Anion exchanger 1 (AE1, band 3) is a major membrane protein of red blood cells and plays a key role in acid-base homeostasis, urine acidification, red blood cell shape regulation, and removal of carbon dioxide during respiration. AE1, a member of the solute carrier ion transport family 4 (SLC4), mediates the exchange of HCO3− with Cl− across plasma membranes. Mammalian erythrocyte AE1 is a ~100 kD integral transmembrane glycoprotein consisting of an N-terminal cytoplasmic domain (CD, residues 1 to 360 in human AE1) and a C-terminal trans-membrane domain (TMD, residues 361 to 911 in human AE1). Here we present the cryoEM structures of full-length bovine AE1 with its TMD captured in both IF and OF conformations.

The classes without CD and fully connected CD are both monomers in IF state. Particles from these two classes were combined and refined using a soft mask of the TM region. The final reconstruction of the IF state was resolved at 4.4 Å. The IF state features an elongated TM11, which incorporates residues from intracellular loop 5 (IL5) between TMs 10 and 11, and partially unfolded TM10. In contrast, the core domain shows a remarkable difference between the OF human and bovine AE1 on one hand and the IF bovine AE1 on the other hand. This difference comes from rigid rotation of the core domain ~20° with respect to the gate domain followed by diagonal downward displacement of the core with <5 Å along the z axis and small lateral motion in the XY plane. Further inspection of the IF structure of bovine AE1 TMD reveals that, due to the rotation and downward motion of the core domain, the ion coordination site becomes open to the cytoplasm and fully closed to the extracellular side, i.e., it is in the IF open state not previously observed in AE1. IL5 between TM10 and TM11, which assumes an antiparallel β-hairpin conformation in the OF state, loses this β-hairpin structure and part of it folds into the elongated α-helix of TM11 in the IF state. The concerted movement of TMs 10 and 11 and the β-hairpin to α-helix transition of IL5 opens a large cavity at the intracellular side and exposes residues R748 and E699 (analogous to residues R730 and E681 in human AE1) to the intracellular solution. At the extracellular side, the downward movement and rotation of TMs 1 and 3 occludes the large permeation cavity seen in the OF state and shields the binding pocket residues I546, F550, E699, and T745-S749 at the previously identified central ion binding site S1 of AE127 from the extracellular solution. The IF conformation is stabilized by several salt bridges between the residues of TMs 1, 3, 5, and 13 (D447-K557, K448-E553, E491-R869), which aid further in the occlusion of the OF cavity.

>MGDPEEYEDQLEETLEQKEYEDHDSVSIPMEEAEGDTIQEEEAEARVNQLTDTDYHTTSQHPETHKVCVQLRELVMDEKNQEIQWMETARWVGLEENLGKDGIWGRPHLPYLNFWSLLELQKAFAKGTVLLDLPGKSLAEVANQLLDRFTFEGQIQPDDQDNLLRVLLLKHSHASDMEALGGVKPVVVTHSGDPSEPLLPQHPSLETELFCEQGEGSTRGHAPEILGKSPQDWEATLVLVGCARFLKRPVLGFVRLKEPMEPEPKPEGSEEPAVPVRFLIVLLGPEGPNINYTQLGRAAATLMSERVFWNDAYLAQSKETLVQSLEGFLDCSLVLPPLDAPSEKALLSLVPVQKELLRRRYLPSPAKPDPSIFKDLDVKKGPGDTPEDPLQRTGKLFGGLVRDIRRRYPRYLSDITDALSPQVLSAIIFIYFAALTPAITFGGLLGDKTENMIGVSELLLSTALQGIIFSLLGAQPLLVLGFSGPLLVFEEAFYSFCQTNNLEYIVGRVWIGFWLILLVVLVVAFEGSFLVRFISRYTQEIFSFLISLIFIYETFYKLVTIFQDHPLQKNYDHDVLTTPKPQAALPNTALLSLVLMAGTFFLAMMLRKFKNSSYFPGKLRRIIGDFGVPISILIMVMVDALIQDTYTQKLSVPEGLSVSNPTERDWLIHPLGIRVEFPIWMMFASALPALLVFILIFLESQITTLIISKPERKMVKGSGFHLDLLLIIGMGGVGAIFGMPWLSATTVRTVTHANALTVMSKDSTPGAVSQIQGVKEQRISGLLVAVLVGVSILMGPVLRHIPLAVLFGIFLYMGVTSLSGIQLFDRVLLLLKPRKYYPEVPYARRVKTWRMHLFTITQIVCLVVLWVVRSIKQISLALPFILILTVPLRRFLLPFIFRDMELKLLDADDVKLNLDEQNGQDEYDEVAMPV[2x]A complex composed of Integrator subunit 3 (Ints3), single-stranded DNA-binding protein 1 (SSB1), and SSB-interacting protein 1 (SSBIP1) is required for efficient homologous recombination-dependent repair of double-strand breaks (DSBs) and ataxia-telangiectasia mutated (ATM)-dependent signaling pathways. Ints3 has an N-terminal and a C-terminal domain connected by a linker region. Ints3 also binds 30-mer random ssDNA and does not bind dsRNA, dsDNA, or DNA/RNA hybrid. Both nucleic acid binding and Ints6 binding properties were attributed to the Ints3 C-terminal domain. Here, we present the crystal structure of the Ints3 C-terminal domain, uncovering a HEAT-repeat superhelical fold.

Finally, in situ proteolysis was used to screen crystals, by adding a trace amount of trypsin in the protein sample (1:1000 w/w). The structure of the human Ints3 C-terminal domain reveals an elongated, HEAT-repeat-like, all α-helical structure. Each repeat is composed of an antiparallel α-helical pair or zigzag, referred to as a- and b-helices. Owing to twists between neighboring repeats, the a- and b-helices form a right-handed α-solenoid. Two copies of the molecule are found in the crystallographic asymmetric unit. Analysis by PISA suggested that a 1702.3 Å2 dimeric surface might be stable and present in solution. Because of the twofold rotational symmetry, helix 6b from molecule A stretches out slightly and sits on top of helices 8b/9b from molecule B, and vice versa. Of these, each of two hydrophobic residues, M780/M781 of helix 6b, sticks into a cavity on the surface of the other molecule. Electrostatic surface analysis of the C-terminal domain dimer revealed an extended groove with a strong positively charged potential.

>[2x]HPIKETVVEEPVDITPYLDQLDESLRDKVLQLQKGSDTEAQCEVMQEIVDQVLEEDFDSEQLSVLASCLQELFKAHFRGEVLPEEITEESLEESVGKPLYLIFRNLCQMQEDNSSFSLLLDLLSELYQKQPKIGYHLLYYLRASKAAAGKMNLYESFAQATQLGDLHTCLMMDMKACQEDDVRLLCHLTPSIYTEFPDETLRSGELLNMIVAVIDSAQLQELVCHVMMGNLVMFRKDSVLNILIQSLDWETFEQYCAWQLFLAHNIPLETIIPILQHLKYKEHPEALSCLLLQLRREKPSEEMVKMVLSRPCHPDDQFTTSILRHWCMKHDELLAEHIKSLLIKNNSLPRKRQSLRSSSSKLAQLTLEQILEHLDNLRLNLTNTKQNFFSQTPILQALQHVQASCDEAHKMKFSDLFSLAEEY> WESKFSKEGLTFDDVLLVPAKSEVLPRDVDLSVELTKTLKLNIPVISAGMDTVTESAMAIAMARQGGLGIIHKNMSIEQQAEQVDKVKRSERGITNPFFLTPDHQVFDAEHLMGKRISGVPIEEDLVGIITNRDLRFISMKISDVMTKEELVTASVGTTLDEAEKILQKHKIEK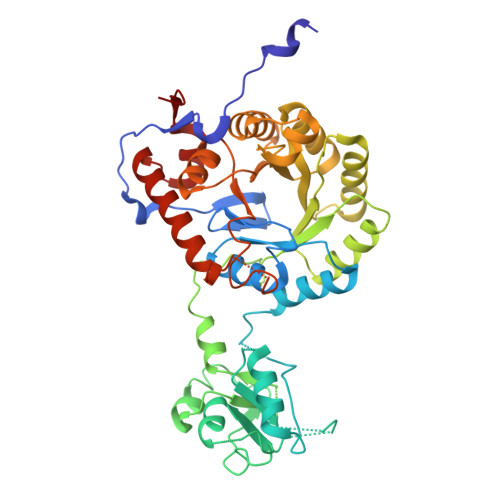LPLVGLITIKDIEKVIEFPNSSKDIHGRLIVGAAVGVTGDTMTRVKKLVEANVDVIVIDTAHGHSQGVLNTVTKIRETYPELNIIAGNVATAEATRALIEAGADVVKVGIGPICTTRVVAGVGVPQITAIYDCATEARKHGKTIIADGGIKFSGDITKALAAGGHAVMLGSLLAGTSESPGETPYKGPVEETVYQLVGGLRSGMGYCGSKDLRALREEAQFIRMTGA> MSVETPSALADSSPHTAPGSAGRSLELGAADIQDLESFEAGRGALPARAYLQSDAPRLSLNGEWQFRLSPGSRVAPDDGWQLGEALNGFESLPVPSSWPMHGHGAPAYTNVQFPFAVEPPHVPEANPIGDHLVVFEAGPEFFPHALLRFDGIESAGTVWLNGVELGTTRGSRLAHEFDVSGILEQGENTLAVRVAQFSAASYVEDQDMWWLPGIFRDVTLQARPAAGIDDVFVHAGYDHITGEGILKVEASRGGQAIDAVVRVPELALELAAGTEVRVPAVEPWSAEVPKLYEAAVSAAGESVALQIGFRSIAIEDAQFKVNGRRILLRGVNRHEHHPRLGRVVPRDVVEAELRLMKQHNINAIRTSHYPPHPQFLALADQLGFYVVLECDLETHGFESAGWAQNPSDDPQWEDALVDRMRRTVERDKNHASVVMWSLGNQAGTGRNLAAMSRWTKDRDPSRPIHYEGDWSSEHVDVYSRMYASQAETALIGQGIEPALNDAALDARRRAMPFVLCEYVHAMGNGPGGMSEYQALFEKYPRLMGGFVWEWLEHGITVSTADGVDHYGYGGDFGEEVHDGNFVTDGLVDADRRPRPGLLDFKKVIEPLRIDVARDWTGFTLRNGQDFADTSAFSFRYEVEADGGALDGGTVDVAPVAPQSETVVELPGSVAALAAGLSDGRPAVLTVRAVLGADSAWADAGHEVAWGQSVREPGAPVPPAPVE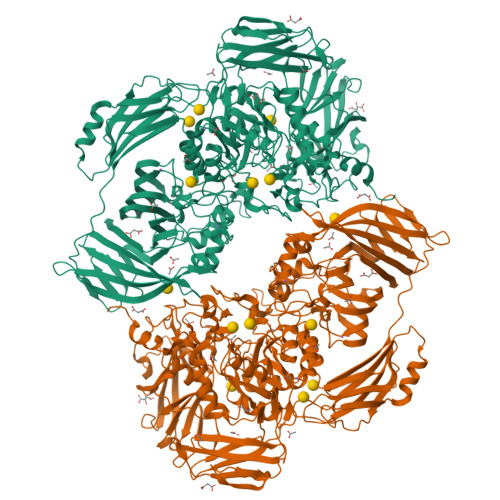PVQVQDSELTLGPVVFSRATGMPTSIGGVPVEKLGLTLWWAPTDNDLGREWGGADERPLATQWKDAGLNRLHTRLLGISANPGQDGGETLTVRTRVSAADKQYGVLVDYTWSTDGETVGLRTQVRRDGTWVNRGFEVEWARIGLEFVLGEETELVSWFGQGPHQSYPDTGQGARAGWFSLPLAKMDVEYVRPQECGARSGSRSAALQLGGRTLEICGDPFALTVRPYSQDVLDAAAHRPDLKADGRTYLYVDHALRGVGTAACGPGVLEQYRLKPRDADFILTLKVRS> SNAESKIKDCPWYDRGFCKHGPLCRHRHTRRVICVNYLVGFCPEGPSCKFMHP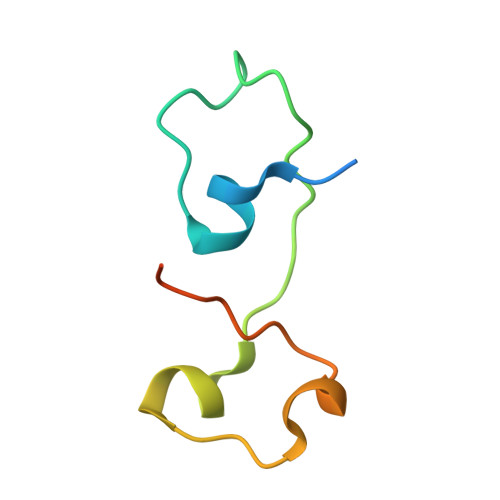RFELPMGTTEQ>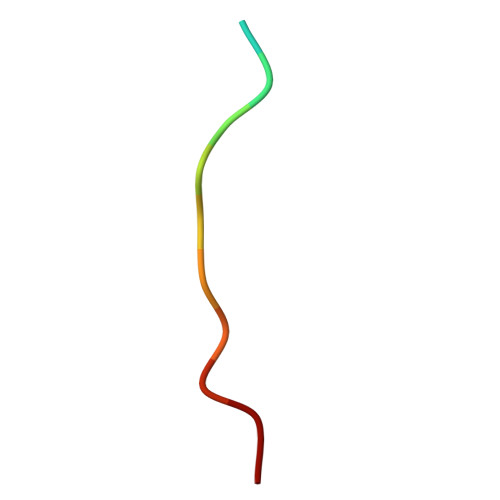 QRPRPTLQLPLA> SNAAIASEFSSLPSYAAFATAQEAYEQAVANGDSEVVLKKLKKSLNVAKSEFDRDAAMQRKLEKMADQAMTQMYKQARSEDKRAKVTSAMQTMLF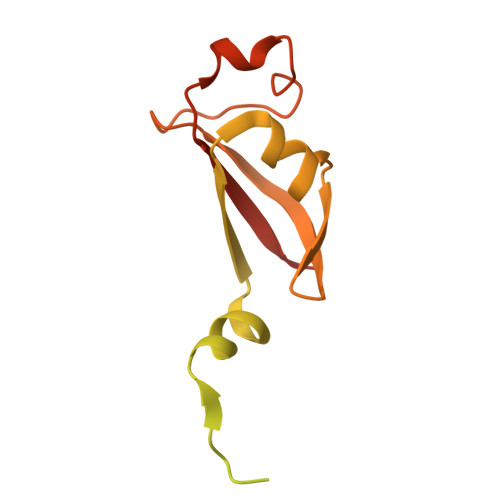TMLRKLDNDALNNIINNARDGCVPLNIIPLTTAAKLMVVIPDYNTYKNTCDGTTFTYASALWEIQQVVDADSKIVQLSEISMDNSPNLAWPLIVTALRANSAVKLQ>[2x]MSKDKGRRYENELVELLKQRGFTAWRVPLSGALGGMFSSDVRVMLAGQE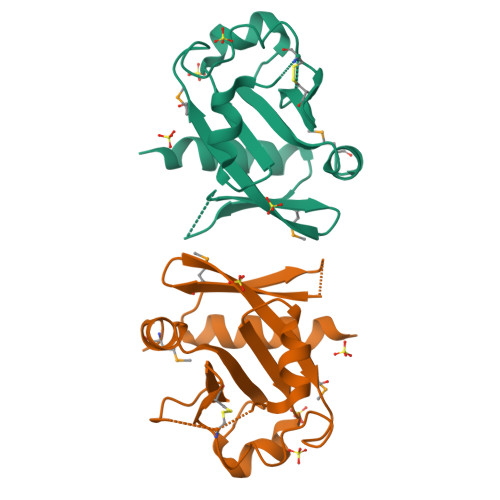HRVEVKMRSTPQAASATRILSKLPFSCQGYRVFFLEALDSQSIMRGEACKKLPKNWVRWLNGAHILAVRLPKRFTSPYGGLTGWIIVLPDTLWDAWRSEMSSDFTGLEHHHHHH>MAHHHHHHSAALEVLFQGPGMASGSNVEEYELDVEALVVILRDRNIPRNPLHGEVIGLRLTEGWWGQIERFQMVRLILQNDDNEPLQRPRYEVIQRAVNPHTMFMISGPLAELQLAFQDLDLPEGPLRFGPLANGHYVQGDPYSSSYRPVTMAETAQMTRDELEDVLNTQSEIEIQMINLLELYEVETRALRRQLAERS[4x];>[4x]MAPPMTLQQWIIWKKMNKAH

PFV Gag is a 648 polypeptide and the major FV structural protein in the assembled virion. Moreover, in all retroviral subfamilies Gag carries out the same functional roles including assembly, nucleic acid packaging, transport to and budding through the cytoplasmic membrane of the producer cell as well as trafficking through the cytoplasm of the target cell and uncoating. Here we report the crystal structure an amino terminal domain from the Gag of PFV (PFV-Gag-NtD), provide the molecular details of the interaction of this domain with the N-terminal leader sequence from the PFV Envelope (PFV-Env) and demonstrate that the PFV-Gag-NtD is also the target for Trim5α restriction factors. Our data reveal that the FV Gag is unique and structurally unrelated to the Gag protein of other retroviruses.

Also unique to FVs is a requirement for the interaction of the Gag protein with the viral envelope protein (Env) in order to bud from the producer cell. It seems likely that FV Gag becomes associated with Env through interaction with Env leader peptide (Env-LP) displayed on the cytosolic side of the ER and Trans-Golgi network (TGN) after core assembly at the pericentriolar region. Env then directs the intracellular transport of the assembled particles to enable mature viruses to bud at the PM or sometimes into intracellular vacuoles. This interaction guarantees Env incorporation into virions and the loss of either interacting domain (Gag-NtD or Env-LP) results in the intracellular stranding of assembled FV capsids. To better understand this interaction and shed light on how FV Gags recruit Env, we examined the interaction of the PFV-Gag-NtD with the PFV-Env-LP using SV-AUC. In the structure, residues 7–16 of the Env leader peptide comprise the amphipathic α-helix bound in the Env binding site of the Gag-NtD and residues 1–6 provide intramolecular hydrogen bonding that stabilises the helical conformation. The affinity of the interaction, 1.5×105 M−1, is comparable with the value of 0.65×105 M−1 reported for the interaction of residues 1–30 of the FFV Env leader peptide with the equivalent Gag-NtD. Therefore, the hydrophobic interface observed in the structure likely represents the complete interaction between the leader peptide and FV Gag. In order to probe the importance of the interactions in the Gag-Env interface observed in the crystal structure a series of serine and asparagine substitutions were introduced at Val14, Leu17, Val18 and Leu21 to make the Env binding site progressively polar. In addition, in order to examine the contribution of the α1-β1 loop to the Env interaction a conservative Asn29 to Gln substitution was also introduced. Mutations in the Env binding site of PFV-Gag-NtD have been shown to affect viral assembly, egress and infectivity.> FSQPFSRPS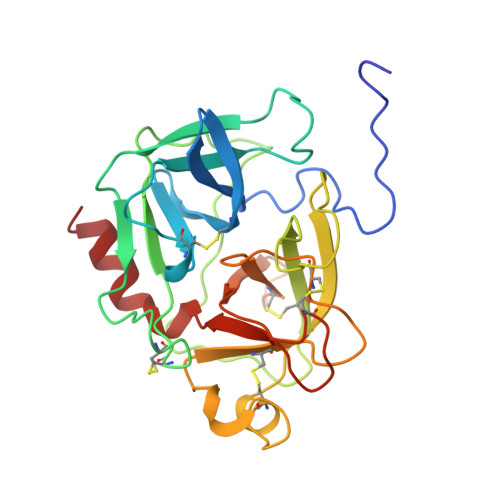SRVVNGEDAVPYSWSWQVSLQYEKDGAFHHTCGGSLIAPDWVVTAGHCISTSRTYQVVLGEYDRSVLQGSEQVIPINAGDLFVHPLWNSNCVACGNDIALVKLSRSAQLGDKVQLANLPPAGDILPNEAPCYISGWGRLYTGGPLPDKLQEALLPVVDYEHCSQYDWWGITVKKTMVCAGGDTRSGCDGDSGGPLNCPAADGSWQVHGVTSFVSAFGCNTIKKPTVFTRVSAFIDWINETIASN>NPAENIASEISKSVEGAIQQVKNLLTLAADRAEQIVNDLASTTTSTITRPIIELSNTADKIAEGNLEAEVPHQNRADEIGI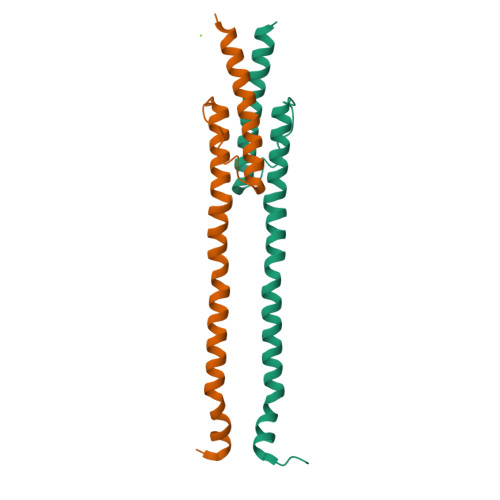LAKSIERLRRSLKVAMESLEEALK[4x]>MQIKAGLIWMNGAFVPQEEAKTSVLSHALHYGTSVFEGIRAYETAKGPAIFRLKEHVKRFYNSAKV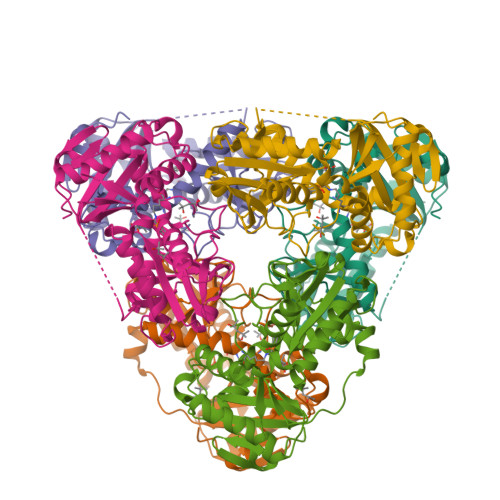LRMEIPFAPEELEEAIKEVVRRNGYRSCYIRPLAWMGAKALGVNPLPNNPAEVMVAAWEWGAYLGEEAVRKGARLITSSWARFPANVMPGKAKVGGNYVNSALAKMEAVAAGADEALLLDEEGYVAEGSGENLFFVRDGVIYALEHSVNLEGITRDSVIRIAKDLGYEVQVVRATRDQLYMADEVFMTGTAAEVTPVSMIDWRPIGKGTAGPVALRLREVYLEAVTGRRPEYEGWLTYVNGQ[3x]> MSEFRIHHDVNELISLLHVFGLEGADVYIDLLQKNRTPYVTTSVSTHSAKVKIAEFSRTPDDFLKKYEELKSKNTRNLDPLVYLLSKLIEDKETLQYLQQNAKDKAELATSSVTSVSLPIAPNTSKISMQELEELRRQLETATVAVSCSHQPVEVLRKFLRDKLNKKHTGHPVPVFPSWVYERPALTGDFMSFSNPSTDVTVSIGTLPLPSQETCLVEDLLYILIGVDGRYISVQPLVGRQSRSFSVEQNLDSSVKELVNRILPVATNYSTVTRFVEENSSFEYGQVNHALGAAMRTLGKEYMILISQLEHLQRQGLLSLQKLWFYIQPTLRTMEVLASIATSLNKGECFGGATLSLLHDRTFGYTGDSQAQELCLYLTKAASAPYFDILERWIYRGIINDPYSEFMVEEHELQKEKIQEDYNDKYWDQRYTIVQQQIPSFLQKVADKILSTGKYLNVVRECGHDVTCPDAKEITYTLKEQAYVERIEKAYNYASKVLLDFLMEEEELVAHLRSIKHYFLMDQGDFFVHFMDLTEEELKKPVDDIIPTRLEALLELALRMSTANTDPFKDDLKIELMPHDLITQLLRVLAIETHQEKALINSDPTELALSGLESFSFDYIVKWPLSLIINRKALTRYQMLFRHMFYCKHVERLLCNVWISNKTAKQFSLHSAKWFAGAFTLRQRMLNFVQNIQYYMMFEVMEPTWHILEKNLKSASNIDDVLSHHTSFLDNCLKDCMLTNPELLKIFSKLMSVCVMFTNCLQRFTQSMQVQTEMEHLTLEHGTMMGPPTQCERTEEALKKKLTSKYLEEHIDKFPSSFGFESTINNFDSNFSAHLMDLLDKLSMYSTSDCEHSMINIIYRLDFNGFYTERLK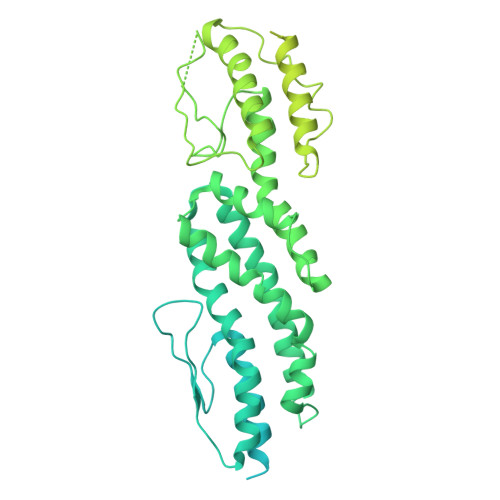QLSSERNQKSAPLLGPAQHAVSTK Non-specific phospholipase C (NPC) hydrolyzes major membrane phospholipids to release diacylglycerol (DAG), a potent lipid-derived messenger regulating cell functions. In contrast, NPC harbors promiscuous activities, hydrolyzing major membrane phospholipids, such as glycosyl inositol phosphoryl ceramide (GIPC), phosphatidylcholine (PC), phosphatidylethanolamine (PE), and phosphatidylserine (PS). NPC4 is divided into a phosphoesterase domain (PD) and a C-terminal domain (CTD), and is structurally distinct from other characterized phospholipases. Mechanistically, CTD contributes NPC4 activity mainly via CTDα1-PD interaction, which ultimately stabilizes the catalytic pocket in PD.

During NPC41–496 crystallization, another set of crystals were obtained after about 2 months. A structure of this crystal was determined at 2.1 Å resolution. Residues encompassing PD (residues 12–258 and 264–415) can be well built in the crystal (NPC41–415), whereas no electron densities (including residues 416–496) are observed for CTD region. Unlike the structure of NPC1–496, no phosphorylation, metal ion and free phosphate molecule occur in this structure. By collecting crystals of the determined NPC41–415 structure, SDS-PAGE results shown that the protein was partially degraded during crystallization, possibly resulting in the omitted CTD in the crystal. Comparing the crystallizing conditions of NPC41–496 and NPC41–415 structures, KH2PO4 was absent in the NPC41–415 crystallization. Superposing the determined structure of NPC41–415 to NPC41–496, the architectures of PD are basically the same but with a significant local conformational change in a loop (including residues 250–268). The catalytic residue H264 in this loop twists out of the catalytic pocket in the NPC41–415 structure (with a measured distance of 8.4 Å), compared to the NPC41–496 structure. Correspondingly, other active site residues are deflected to a certain extent. It showed that the substrate hydrolyzing-activity of NPC41–415 was almost eliminated.

>[2x]MIETTKGGSGSYPIKTIVVLVQENRSFDHTLGWFKELNREIDGVTKSDPKSNTVSSSDTNSLRVVFGDQSQYVNPDPGHSIQDIYEQVFGKPWDSGKPDPNPGHPNMSGFAQNAERNKKGMSSAVMNGFKPNALPVYKELVQNFAICDRWFASVPASTQPNRLYVHSATSHGATSNDAALLLEGFPQKTIFESLDEAGFSFGIYYQFPPSTLFYRNLRKLKYLTHFHQYGIQFKKDCKEGKLPNYVVVEQRWFDLLSTPANDDHPSHDVSEGQKLVKEVYEALRSSPQWNEILFIITYDEHGGFYDHVPTPVDGVPNPDGILGPPPYNFEFNRLGVRVPTFFISPWIEPGTVIHGPNGPYPRSQYEHSSIPATVKTIFKLKDFLSKRDSWAGTFESVITRDSPRQDCPETLSTPIKLRGTMAKENAQLSEFQEDLVIMAAGLKGDYKNEELIHKLCKETCVADASKYVTNAFEKFLEESRKARDRGCDENDIVY>[2x]MDDLDLPDPSLKNIIDQTTLQWVFVGGKGGVGKTTTSCCLGVQLAKSRTKVLLVSTDPAHNLSDAFCQKIGREPTPIHGFDNLCAMEIDASQEAESEIEATDDNDVFGQMFNDLQNSIPGIDEAMSFSELMKQVQQLDFD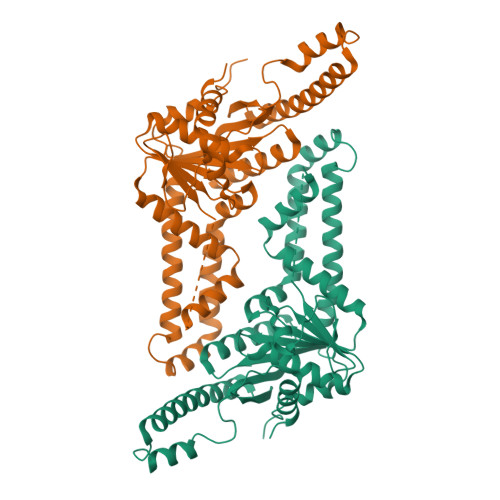VVVFDTAPTGHTLRLLSFPTILEKAFAKVWELKDRFGGLIGQATALMSGGNNPAAAQEQLLGKLEETRAVINKVNQAFQDPTKTTFVCVCIPEFLSIYETERLVQELSKYGIDSHNIVVNQVLFPEKDAEELSAWYEANGATLPKEAREICSKLLARKRMQDKYIGQCFDLYGDDFHVVLMPLLDYEVRGVEKLKTFSELLVDPVDMDE> MSEVFQECVNLFIKRDIKDCLEKMSEVGFIDITVFKSNPMILDLFVSACDIMPSFTKLGLTLQSEILNIFTLDTPQCIETRKIILGDLSKLLVINKFFRCCIKVIQFNLTDHTEQEEKTLELESI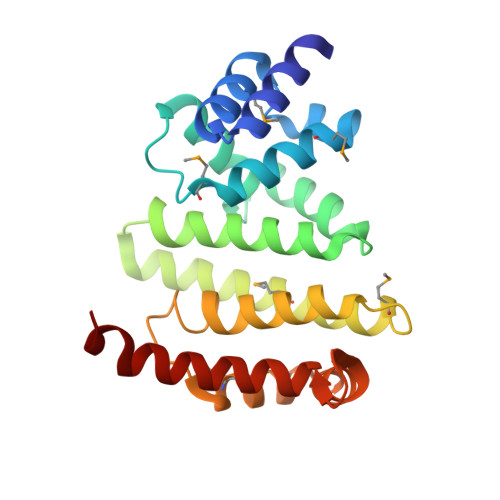MSDFIFVYITKMRTTIDVVGLQELIEIFIFQVKVKLHHKKPSPNMYWALCKTLPKLSPTLKGLYLSKDVSIEDAILNSIDNKIQKDKLEVLFQ>VPRGSHMSNEAHTLVTPEGNVIDIQGASQENGANAIIYPRHGGENQLFFIDKQIGWIISVFSRKALTVKENMHDIVQSDYCSLSRQQWIFEDNPDGTTIIRCYENPELVLSVTGNIDKVCLSPFTREAHQLWRI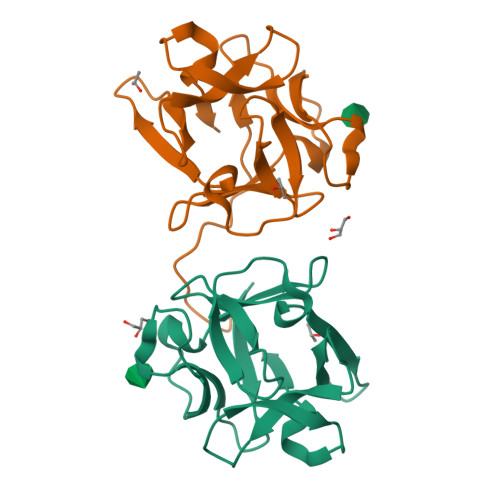E[2x]>[2x]STMGL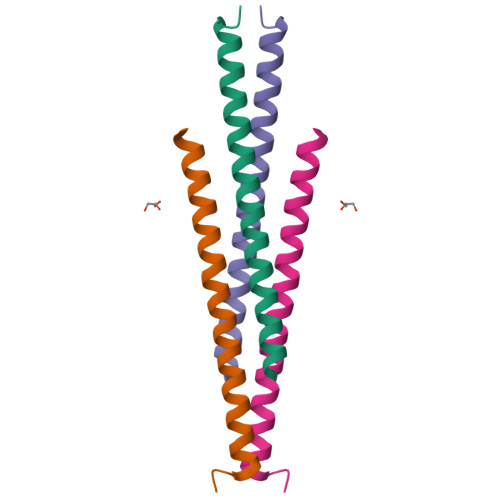LSQENTQIRDLQQENRELWISLEEHQDALELIMSKYRKQMLQLMVAKKA Soluble HMW1C-like N-glycosyltransferases (NGTs) catalyze the glycosylation of Asn residues in proteins, a process fundamental for bacterial autoaggregation, adhesion and pathogenicity. In contrast, NGTs are two-domain enzymes that consists of an N-terminal all-α domain (AAD) and a C-terminal catalytic domain that adopts a GT-B fold, as shown for Actinobacillus pleuropneumoniae NGT (ApNGT). We focused on AaNGT, an inverting GT that catalyzes the transfer of Glc from UDP-Glc to Asn residues in the consensus sequence Asn-X-Ser/Thr. The heart-shaped structure of AaNGT, either complexed to UDP-Gal/UDP-2F-Glc or UDP-peptide, shows the N-terminal AAD domain and C-terminal GT-B fold catalytic domain, which is composed of an N- and C-Rossman fold subdomains.

We provide high-resolution crystal structures for the enzyme in complex with a poor donor substrate (UDP-Gal) and a donor mimic (UDP-2F-Glc), as well as the enzyme in complex with a peptide acceptor (FGNWTT) and UDP, together with kinetic/ITC experiments and QM/MM metadynamics simulations of the reaction mechanism. We used 500 µM concentrations of the sugar nucleotides and the peptide (saturated conditions found for UDP-Glc and the peptide), and found that the initial velocity with UDP-Gal was ~40-fold lower than that of UDP-Glc and completely inactive with either UDP-2F-Glc or UDP-5S-Glc, implying that we could potentially trap co-crystals of AaNGT complexed to UDP-Glc mimetics and the peptide. In contrast, the UDP-Gal and UDP-2F-Glc pyrophosphates are only recognized by the side chains of Lys440 and Asn520. The sugar molecules interact with the side chains of His276 and Ser277. Furthermore, the Gal moiety specifically interacts with the Gly369 backbone, while the 2F-Glc moiety interacts with the side chain of His370. The superposition of all ligands for all three structures (AaNGT/UDP, AaNGT/UDP-Gal, and AaNGT/UDP-2F-Glc) clearly shows that the sugar moieties of UDP-Gal and UDP-2F-Glc collide with Gly2-1 and Asn30. This suggests that the sugar nucleotides adopt unproductive conformations in their respective enzyme complexes, which could explain why we were unable to get a ternary complex resembling a Michaelis complex at a structural level. Furthermore, this could also explain why UDP-Gal is a poor substrate, and UDP-Glc mimetics are inhibitors of AaNGT. The interaction of the 2-OH and the β-phosphate group could explain why the enzyme cannot recognize UDP−2F-Glc in a productive manner. Diffraction was poor for crystals obtained in the presence of UDP-5S-Glc, thus precluding obtaining useful data with this sugar nucleotide. Attempts to obtain a ternary complex that resembles a Michaelis complex by combining the UDP-2F-Glc or UDP-Gal with the peptide yielded a complex without peptide (see below for an explanation).

>[2x]GMSRKKNPSVIQFEKAITEKNYEAACTELLDILNKIDTNFGDIEGIDFDYPQQLETLMQDRIVYFCTRMSNAITQLFCDPQFSLSESGANRFFVVQRWLNLIFASSPYINADHILQTYNCNPERDSIYDIYLEPNKNVLMKFAVLYLPESNVNLNLDTMWETDKNICGSLCFALQSPRFIGTPAAFSKRSTILQWFPAKLEQFHVLDDLPSNISHDVYMHCSYDTAENKHNVKKALNQVIRSHLLKCGWQDRQITQIGMRNGKPVMVVVLEHFHSSHSIYRTHSTSMIAAREQFYLIGLGNNAVDQAGRDVFDEFHEFDGSNILKKLAFLKEMCEKNDAAVLYMPSIGMDLATIFVSNARFAPIQVIALGHPATTHSEFIEYVIVEDDYVGSESCFSETLLRLPKDALPYVPSSLAPTDVQYVLRETPEVVNIGIAATTMKLNPYFLETLKTIRDRAKVKVHFHFALGQSIGITHPYVARFIRSYLGDDATAHPHSPYNRYLDILHNCDMMLNPFPFGNTNGIIDMVTLGLVGVCKTGPEVHEHIDEGLFKRLGLPEWLIADSVEDYIERAIRLAENHQERLALRRHIIENNGLKTLFSGDPSPMGKTLFAKLTEWRQTNGI>[2x]MGSSHHHHHHSSGETVRFQGHMNLSQLSFHRVDQKEITQLSHLGQGTRTNVYEGRLRVEGSGDPEEGKMDDEDPLVPGRDRGQELRVVLKVLDPSHHDIALAFYETASLMSQVSHTHLAFVHGVCVRGPENIMVTEYVEHGPLDVWLRRERGHVPMAW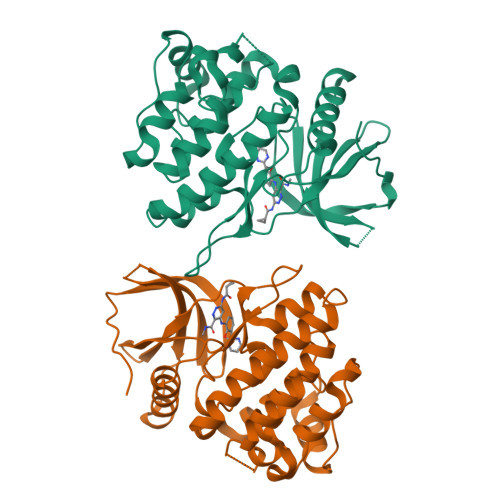KMVVAQQLASALSYLENKNLVHGNVCGRNILLARLGLAEGTSPFIKLSDPGVGLGALSREERVERIPWLAPECLPGGANSLSTAMDKWGFGATLLEICFDGEAPLQSRSPSEKEHFYQRQHRLPEPSCPQLATLTSQCLTYEPTQRPSFRTILRDLTRL> SSRFESLFAGEKE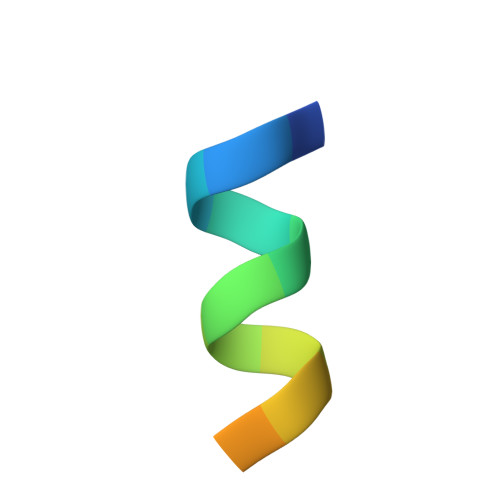SR> SLLNVPAGKDLPEDIYVVIEIPANADPIKYEIDKESGALFVDRFMSTAMFYPCNYGYINHTLS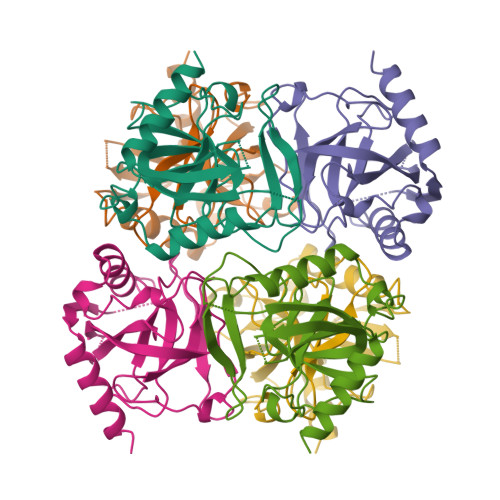LDGDPVDVLVPTPYPLQPGSVIRCRPVGVLKMTDEAGEDAKLVAVPHSKLSKEYDHIKDVNDLPELLKAQIAHFFEHYKDLEKGKWVKVEGWENAEAAKAEIVASFERAKNK>MNLPTAQEVQGLMARYIELVDVGDIEAIVQMYADDATVENPFGQPPIHGREQIAAFXRQGLG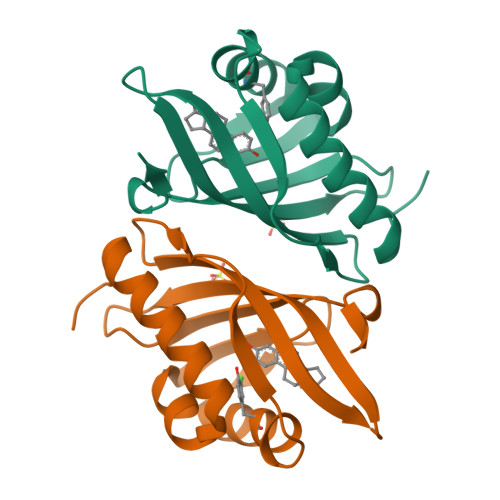GGKVRACLTGPVRASHNGCGAMPFRVEMVWNGQPCALDVIDVMRFDEHGRIQTMQAYWSEVNLSVREPQLVPR[2x]Investigation of bat, rat and musk shrew samples from within the cave, where the victims had most probably contracted the disease, led to the discovery of a novel rat-borne paramyxovirus, Mòjiāng virus (MojV)1. Analysis of the MojV genome reveals that the paramyxovirus is closely related to viruses within the genus Henipavirus, an emergent zoonotic group of bat-borne pathogens distributed throughout Asia, Australia, Central America and Africa. Viral attachment is a primary determinant of host cell tropism and is initiated by a haemagglutinin-neuraminidase (HN) glycoprotein, haemagglutinin (H) glycoprotein or attachment (G) glycoprotein, depending on the virus. Although MojV-G displays a six-bladed β-propeller fold characteristic to paramyxoviral attachment glycoproteins, our analyses also show that MojV-G is antigenically, structurally and functionally distinct from all other characterized paramyxoviruses.

A construct encoding some residues from the putative MojV-G stalk region (residues 166–193), the β-propeller domain (residues 194–605) and the C-terminal extension (residues 606–625), was expressed in HEK 293T cells in the presence of an α-mannosidase inhibitor, kifunensine. Following deglycosylation with endoglycosidase F1 (EndoF1), MojV-G was crystallized and the structure was determined to 1.94 Å resolution. MojV-G exhibits a six-bladed β-propeller fold, characteristic of Paramyxovirinae attachment glycoproteins, with each blade of the propeller composed of four antiparallel β-strands. The β-propeller fold is stabilized by seven disulfide bonds, all of which are conserved among HNVs. Two nearly identical molecules of MojV-G were observed in the asymmetric unit (0.33 Å root-mean-square (RMS) deviation over 412 aligned Cα atoms), although crystallographic contacts were not consistent with the formation of higher-order MojV-G oligomers, such as those observed in HeV-G18 or other paramyxoviruses. However, a portion of the crystallized N-terminal stalk region was clearly visible (residues 175–193) and folds underneath the sixth blade of the β-propeller domain in a conformation analogous to that observed in full-length Newcastle disease virus (NDV) HN glycoprotein and parainfluenza 5 HN (PIV5-HN) glycoprotein ectodomain structures. Unlike other paramyxovirus attachment glycoproteins, which are glycosylated throughout the β-propeller18192021222324353637383940414243444546, the ectodomain of MojV-G encodes only four N-linked glycosylation sequons, all of which are located outside the β-propeller domain. Indeed, we observe that paramyxoviral receptor-interacting surfaces exhibit some of the greatest levels of structural deviation with respect to MojV-G. For example, the top face of the MojV-G β-propeller lacks the distinctive ephrin binding pocket observed in NiV-G and other HNVs, and exhibits very low sequence conservation with other HNVs at this region.

>TGDTTDDDKVDTTIKPIEYPKPDGCNRTGDHFTMEPGANFYTVPNLGPASSNSDECYTNPSFSIGSSIYMFSQEIRKTDCTAGEILSIQIVLGRIVDKGQQGPQASPLLVWAVPNPKIINSCAVAAGDEMGWVLCSVTLTAASGEPIPHMFDGFWLYKLEPDTEVVSYRITGYAYLLDKQYDSVFIGKGGGIQKGNDLYFQMYGLSRNRQSFKALCEHGSCLGTGGGGYQVLCDRAVMSFGSEESLITNAYLKVNDLASGKPVIIGQTFPPSDSYKGSNGRMYTIGDKYGLYLAPSSWNRYLRFGITPDISVRSTTWLKSQDPIMKILSTCTNTDRDMCPEICNTRGYQDIFPLSEDSEYYTYIGITPNNGGTKNFVAVRDSDGHIASIDILQNYYSITSATISCFMYKDEIWCIAITEGKKQKDNPQRIYAHSYKIRQMCYNMKSATVTVGNAKNITIRRYGTKHHHHHH[2x]> MGALESLRGNADLAYILSMEPCGHCLIINNVNFCRESGLRTRTGSNIDCEKLRRRFSSLHFMVEVKGDLTAKKMVLALLELARQDHGALDCCVVVILSHGCQASHLQFPGAVYGTDGCPVSVEKIVNIFNGTSCPSLGGKPKLFFIQACGGEQKDHGFEVASTSPEDESPGSNPEPDATPFQEGLRTFDQLDAISSLPTPSDIFVSYSTFPGFVSWRDPKSGSWYVETLDDIFEQWAHS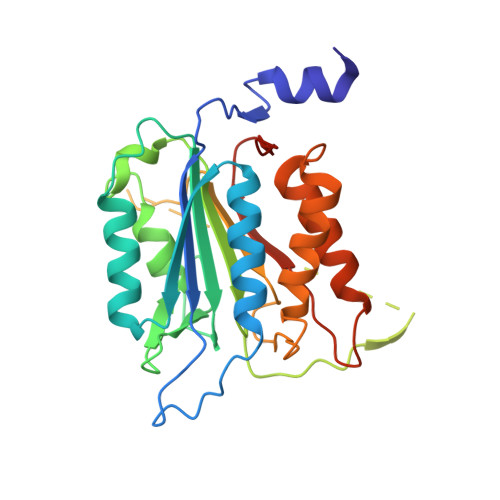EDLQSLLLRVANAVSVKGIYKQMPGCFNFLRKKLFFKTSHHHHHH>LHLTQPQILFVRKTWNHARNQGALEPAISIFRNSFFKNPEIRQMIMFGTKNEGHERLKKHAQLFTVLMDDLIANLDSPSATVAGLREAGEKHVWPTRNQYGCPFHAHLLDQFATAMIERTLEWGEKKDRTETTQRGWTKIV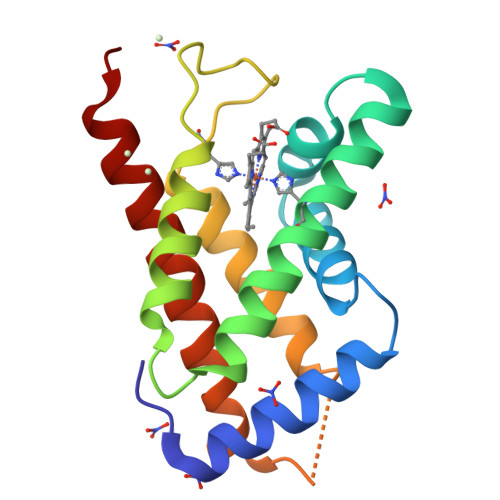LFVTEQLKEGFQDEQKRARR[2x]>[6x]MELYLIRHGIAEAQ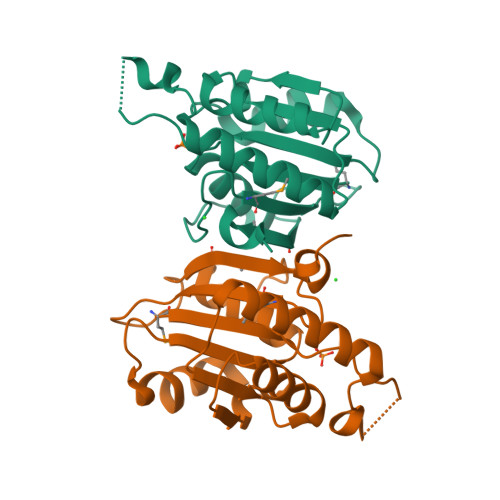KTGIKDEERELTQEGKQKTEKVAYRLVKLGRQFDLIVTSPLIRARQTAEILLASGLSCQLEESNHLAPNGNIFNWLDYWLKPKNFPENAQIAIVGHEPCLSNWTEILLWGEAKDSLVLKKAGMIGLKLPEIGSPVGRSQMFWLTPPRYLLLEHHHHHH>[12x]MAKAVDAAAAAAAAIAPVDTTVVNEDVALVENETCNDQNVQFDSLPSMKYASFLNSDGSVAIHAGERLGRGIVTDAITTPVVNTSAYFFNKTSELIDFKE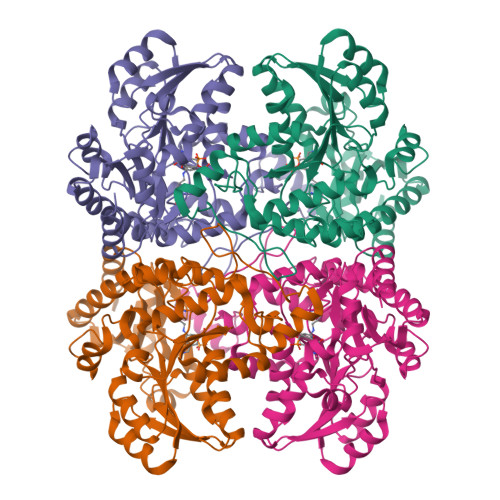KRRASFEYGRYGNPTTVVLEEKISALEGAESTLLMASGMCASTVMLLALVPAGGHIVTTTDCYRKTRIFIETILPKMGITATVIDPADVGALELALNQKKVNLFFTESPTNPFLRCVDIELVSKLCHEKGALVCIDGTFATPLNQKALALGADLVLHSATKFLGGHNDVLAGCISGPLKLVSEIRNLHHILGGALNPNAAYLIIRGMKTLHLRVQQQNSTALRMAEILEAHPKVRHVYYPGLQSHPEHHIAKKQMTGFGGAVSFEVDGDLLTTAKFVDALKIPYIAPSFGGCESIVDQPAIMSYWDLSQSDRAKYGIMDNLVRFSFGVEDFDDLKADILQALDSI> GIEETIDTVITNALQLSQPKPQKQPTAQSTPLTSGVNSQEVPALTAVETGASGQAVPSDVIETRHVVNYKTRSESTLESFFGRSACVTILEVENFNATTDADRKKQFTTWAITYTDTVQLRRKLEFFTYSRFDLEMTFVITERYYASNTGHARNQVYQLMYIPPGAPRPTAWDDYTWQSSSNPSVFYTYGSAPPRMSIPYVGIANAYSHFYDGFARVPLKDETVDSGDTYYGLVTINDFGTLAVRVVNEYNPARITSKIRVYMKPKHVRCWCPRPPRAVPYRGEGVDFKQD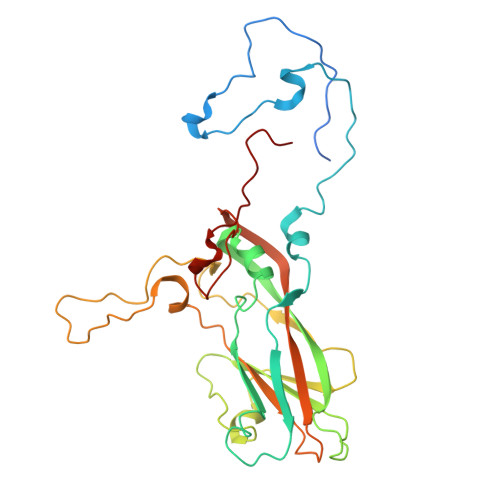SITPLTAVENINTF The Src homology 3 (SH3) domain is a ∼60-residue modular domain that consists of two antiparallel β-sheets orthogonally packed to form a single hydrophobic core. This domain is present in many proteins and regulates critical cellular pathways by recognizing polyproline-rich motifs (PRMs; Kurochkina & Guha, 2013). Three-dimensional domain swapping (3D-DS) is a mechanism by which some proteins can oligomerize by exchanging identical domains or structural elements between monomers. In previous work, the 3D-DS of the c-Src SH3 domain has been characterized and its dependence on experimental conditions has been described. This work explores the role of the hinge-loop composition by interchanging residues in the RT and n-Src loops between two SH3 domains: one being the c-Src SH3 domain, where 3D-DS has been described, and the other being the Abl SH3 domain, where 3D-DS has not been described to date.

However, the interchange of one or two loops within the Abl SH3 domain produces a noticeable reduction in its stability but does not promote the formation of 3D domain-swapped oligomers. Conversely, replacing the RT and n-Src loop residues in the Abl_Src chimeras with those from the c-Src SH3 domain results in destabilization under identical denaturing conditions. Notably, the Abl_Src-nSrc and Abl_Src-2 chimeras exhibit pronounced destabilization, highlighting a key role for the c-Src n-Src loop residues in determining the stability of these chimeric proteins. In this way, the ΔG values are the same for the WT and Abl_Src-RT, but the Abl_Src-nSrc and Abl_Src-2 chimeras show a noticeable loss of stability. However, Src_Abl-nSrc shows an ordered distal loop in most of the molecules in the asymmetric unit and this chimera does not form the intertwined dimer. The same behaviour can be observed in the Abl_Src chimeras, where the distal loop shows low B factors. Indeed, even though the Abl_Src chimeras are less stable, this reduction in stability does not allow formation of the intertwined dimer.

>[2x]GPNLFVALYDFESRTENTLSITKGEKLRVLNNTENGEWCEAQTKNGQGWVPSNYITPVN>HHHHHHGSMALYGFAQGLIQEAGIRIKQLMEQNLTIETKSNPNDLVTNVDKATEDFIFDTILETYPNHQVLGEEGHGHDIDTSKGTVWVVDPIDGTLNFVHQQENFAISIGIYIDGKPYAGFVYDVMADVLYHAKVGEGAYRGSQPLKPLNDSNLRQSIIGINPNWLTKPILGEIFKEIVNDSRSARAYGSAALEIVSVATGNLEAYMTPRLQPWDFAGGLVILYEVNGQASNLLGEPLTISGPNSILVGNRGLHQEISND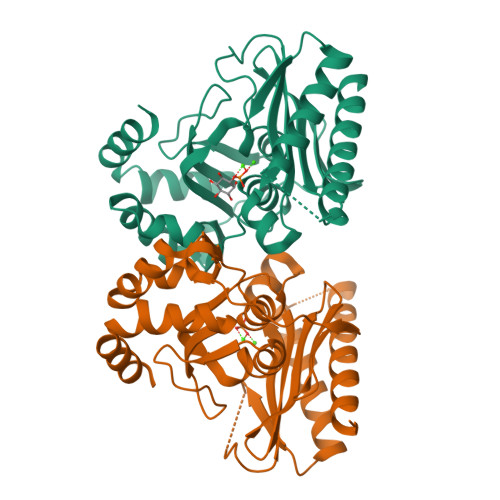YLEPHHDALIQLHEQRFKRKSK[4x]>PNFSGNWKIIRSENFEELLKVLGVNVMLRKIAVAAASKPAVEIKQEGDTFYIKTSTTVRTTEINFKVGEEFEEQTVDGRPCKSLVKWESENKMVCEQKLLKGEGPKTSWTRELTNDGELIETMTADDVVCTKVYVR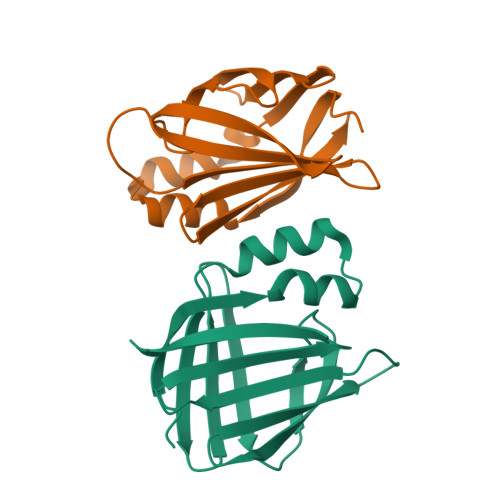E[2x]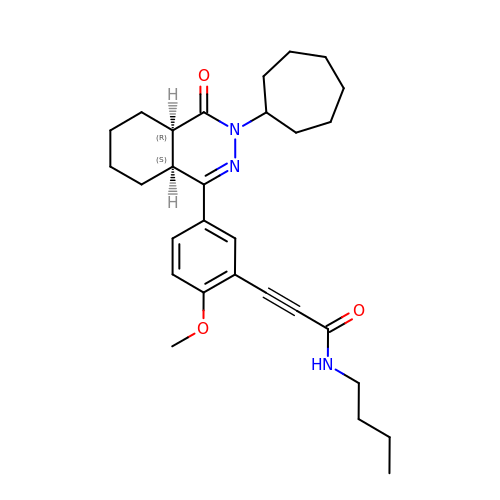3-[5-[(4~{a}~{R},8~{a}~{S})-3-cycloheptyl-4-oxidanylidene-4~{a},5,6,7,8,8~{a}-hexahydrophthalazin-1-yl]-2-methoxy-phenyl]-~{N}-butyl-prop-2-ynamide | C29 H39 N3 O3 | QLHBWGPAEHWNOH-LOSJGSFVSA-N2-[3-(tetrahydro-2H-pyran-4-yloxy)propyl]-1,2,3,4-tetrahydroisoquinolin-8-amine | C17 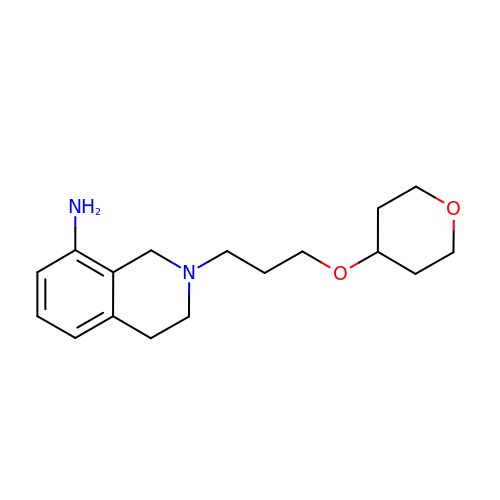H26 N2 O2 | XCARWFGYJXOJRR-UHFFFAOYSA-N>[4x]CGPKRDPYAKAGKSEGKPDKLVVWENADDGVQLNNTKKWAGEFTKKTGIQVEVVPVALLKQQEKLTLDGPAGKGADLVTWPHDRLGEAVTKGLLQPIQVDNSVKNQFDDVAMKALTYGGKLYGLPKAIESVALIYNKKLMGQVPATYDELFQYAKANNKPDEQKYGVLFEANNFYYTYFLFAAKGAAVFKEQDGTLDPNEIGLNSPEAVQGMNEVQKWFTEARLPQSLK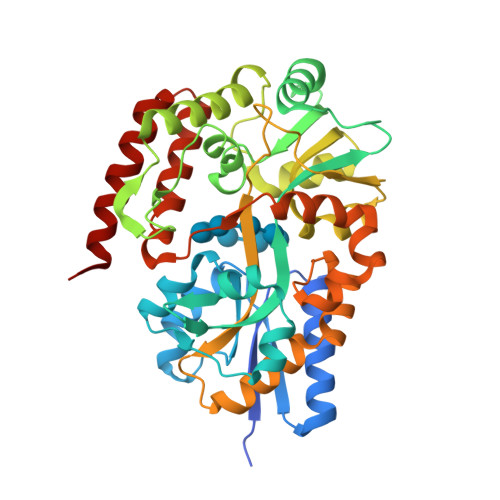ADTVNGLFKSGKVAAVINGPWAIKDYQAAGINVGVAPLPKIDGKDAQTFIGVKGWYLSAYSKYPKYATELMQFLTSKEALASRFKETGEIPPQKELLNDPMIKNNPVVNGFAKQASKGVPMPSIPEMGVVWEPINNAHTFVAQGKQTPEQALNDAVKIMKEKIQTMKQ>[2x]PQYQTWEEFSRAAEKLYLADPMKARVVLKYRHSDGNLCVKVTDDLVSLVYKTDQAQDVKKIEKFHSQLMRLMVAKEARNVTMETE;>[2x]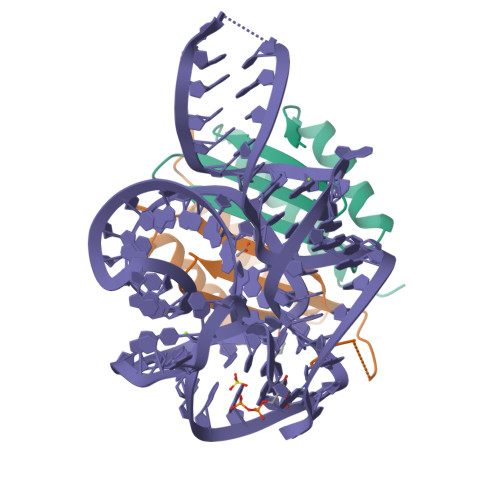GAMESEQFLTELTRLFQKCRTSGSVYITLKKYDGRTKPIPKKGTVEGFEPADNKCLLRATDGKKKISTVVSSKEVNKFQMAYSNLLRANMDGLK> SNANKSAGTQAEKTATDLPPGFSGKAGSANATPGTKGLDGPTPLADGSFDATIFGPAKELKSADDILNVHRRNAKDPF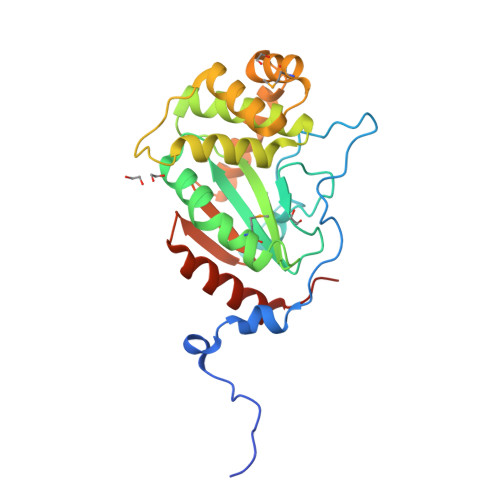AVGAVDAPLVITEFSDFECPFCARWSNQTEPTLMEEYVSKGLVRIEWNDLPVNGEHALAAAKAGRAAAAQGKFDEFRKALFEASRNVSGHPNNTLKDFERFARNAGVKDMERFSREAQDSTYDEVLTKAADYAHGLGVSGTPAFVVGTQYISGAQPTEEFIKVIESELKKSPTFSTPSSHQN> MEI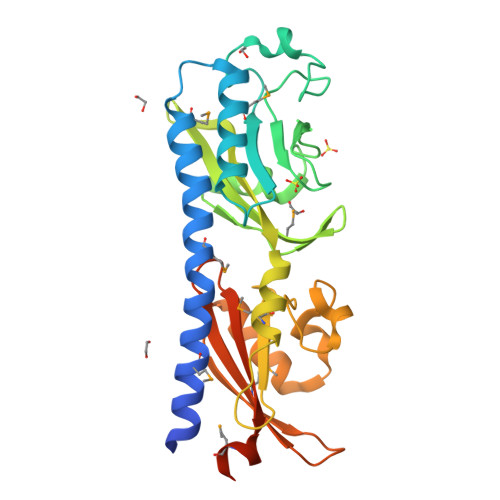GTVTSQEEKLAYEKSIEMAGNYANQFDAQMEANQAIARTLACTMAEYGSQDREEAMSIIKRILNENPQLIGVYLGYEPDAFDGRDKNYINAPGHDSTGRFVPYCNKINGPVIIEPLVHYDSSDYYQLPKTTGKDTLTEPYFYEGIFMVSYDSPIFKNGEFAGIAGVDVPLEYVDDVASSIRTFDTGYAFMVSNTGIFLSHPTQKNWIGEKSLSDFDVEEIKNAASDIREGIGGHVEIKDPITGKTVIMFYEPVKTGDFSFVLVVPKEEMLAGVKDLRDRLLEHHHHHH>[2x]METRTLEDWRALLEAEKTLDSGVYNKHDLLIVRGQGARVWDAEGNEYIDCVGGYGVANLGHGNPEVVEAVKRQAETLMAMPQTLPTPMRGEFYRTLTAIL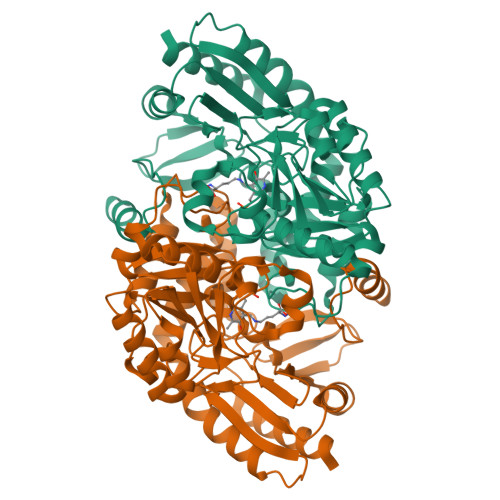PPELNRVFPVNSGTEANEAALKFARAHTGRKKFVAAMRGFSGRTMGSLSVTWEPKYREPFLPLVEPVEFIPYNDVEALKRAVDEETAAVILEPVQGEGGVRPATPEFLRAAREITQEKGALLILDEIQTGMGRTGKRFAFEHFGIVPDILTLAKALGGGVPLGVAVMREEVARSMPKGGHGTTFGGNPLAMAAGVAAIRYLERTRLWERAAELGPWFMEKLRAIPSPKIREVRGMGLMVGLELKEKAAPYIARLEKEHRVLALQAGPTVIRFLPPLVIEKEDLERVVEAVRAVLA>MQLNNRDLKSIIDNEALAYAMYTVENRAIPNMIDGFKPVQRFVIARALDLARGNKDKFHKLASIAGGVADLGYHHGENSAQDAGALMANTWNNNFPLLDGQGNFGSRTVQKAAASRYIFARVSKNFYNVYKDTEYAPVHQDKEHIPPAFYLPIIPTVLLNGVSGIATGYATYILPHSVSSVKKAVLQALQGKKVTKPKVEFPEFRGEVVEIDGQYEIRGTYKFTSRTQMHITEIPYKYDRETYVSKILDPLENKGFITWDDACGEHGFGFKVKFRKEYSLSDNEEERHAKIMKDFGLIERRSQNITVINEKGKLQVYDNVVDLIKDFVEVRKTYVQKRIDNKIKETESAFRLAFAKAHFIKKVISGEIVVQGKTRKELTEELSKIDMYSSYVDKLVGMNIFHMTSDEAKKLAEEAKAKKEENEYWKTTDVVTEYTKDLEEIKHHHHHHHHHH[2x];>[2x]MIKNEIKILSDIEHIKKRSGMYIGSSANEMHERFLFGKWESVQYVPGLVKLIDEIIDNSVDEGIRTKFKFANKINVTIKNNQVTVEDNGRGIPQAMVKTPTGEEIPGPVAAWTIPKAGGNFGDDKERVTGGMNGVGSSLTNIFSVMFVGETGDGQNNIVVRCSNGMENKSWETIPGKWKGTRVTFIPDFMSFETNELSQVYLDITLDRLQTLAVVYPDIQFTFNGKKVQGNFKKYARQYDEHAIVQEQENCSIAVGRSPDGFRQLTYVNNIHTKNGGHHIDCVMDDICEDLIPQIKRKFKIDVTKARVKECLTIVMFVRDMKNMRF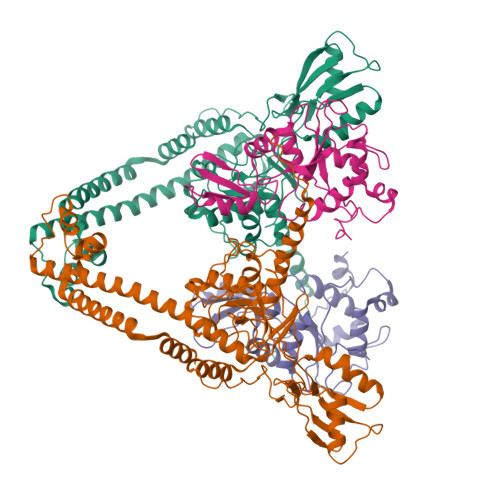DSQTKERLTSPFGEIRSHIQLDAKKISRAILNNEAILMPIIEAALARKLAAEKAAETKAAKKASKAKVHKHIKANLCGKDADTTLFLTEGDSAIGYLIDVRDKELHGGYPLRGKVLNSWGMSYADMLKNKELFDICAITGLVLGEKAENLNYHNIAIMTDADHDGLGSIYPSLLGFFSNWPELFEQGRIRFVKTPVIIAHVGKKQEWFYTVAEYESAKDALPKHSIRYIKGLGSLEKSEYREMIQNPVYDVVKLPENWKELFEMLMGDNADLRKEWMSQHHHHHH>MDHLPIFCQLRDRDCLIVGGGDVAERKARLLLEAGARLTVNALTFIPQFTVWANEGMLTLVEGPFDETLLDSCWLAIAATDDDTVNQRVSDAAESRRIFCNVVNAPKAASFIMPSIIDRSPLMVAVSAGGTSPVLARLLREKLESLLPQHLGQVARYAGQLRARVKKQFATMGERRRFWEKFFVNDRLAQSLANADEKAVNATTERLFSEPLDHRGEVVLVGAGPGDAGLLTLKGLQQIQQADIVVYDRLVSDDIMNLVRRDADRVFVGKRAGYHCVPQEEINQILLREAQKGKRVVR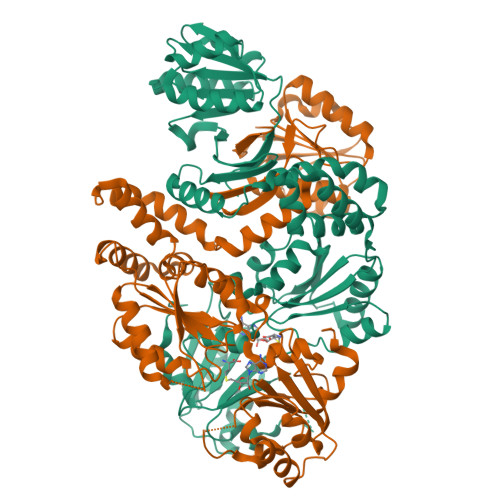LKGGDPFIFGRGGEELETLCHAGIPFSVVPGITAASGCSAYSGIPLTHRDYAQSVRLVTGHLKTGGELDWENLAAEKQTLVFYMGLNQAATIQEKLIAFGMQADMPVALVENGTSVKQRVVHGVLTQLGELAQQVESPALIIVGRVVALRDKLNWFSNH[2x]(5R,6R,7S,8R)-5-(HYDROXYMETHYL)-5,6,7,8-TETRAHYDROIMIDAZO[1,2-A]PYRIDINE-6,7,8-TRIOL 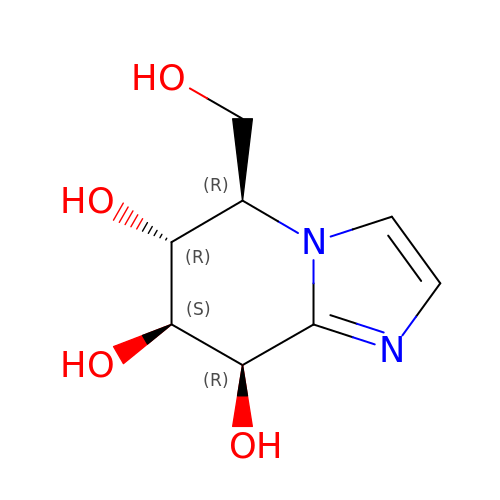| C8 H12 N2 O4 | RZRDQZQPTISYKY-JWXFUTCRSA-N> GIDPFTSTQQHTEPAEEETLHNIITDTENVQGSFSKHEFQAETKKLLDIVARSLYSEKEVFIRELISNGSDALEKLRHRMITAGGDTAPMEIHLQTDSVKGTFTIQDTGVGMNKEDLVSNLGTIARSGSKAFLDALQNQAEASSSIIGQFGVGFYSAFMVADKVEVYSQSAEADAPGYKWSSDGSGVFEVAEASGVRQGTKIVLHLKDDCKEFSSEDRVKEVVTKYSNFVSFPIFLNGRRLNTLQALWMMEPKDISEWQHEEFYRYVAQAYDKPRYTLHYRADAPLNIRSIFYVPEMKPSMFDVSREMGSSVALYSRKILIQTKATDILPKWLRFLRGVVDSEDIPLNLSRELLQESALIRKLRDVLQQRVIRFLLDQSKKDPEKYARFFEDYGLFMREGIVTTGEQSVKEDIAKLLRFESSALPAGQQTSLMEYSSRMKAGTRNIYYLCAPNRHLAEHSPYFEAMKQKDMEVLFCFEQFDELTLLHLREFDRKKLISAETDIVVDHYKEEKFQDSKPASERLSSEQAEDLLAWMRNALVQRVTNIKVTPRLDTHPAMITVLEMGAARHFLRTQQLARSSEERAQILQPTLEINTGHDLIKKLHALKDSNPELAQLLLEQIYDNAMIAAGLNEDPRPMISRLNQLLTRALEKHGSDSATHIKFSKRDEDGKELAGATMELRDSSGK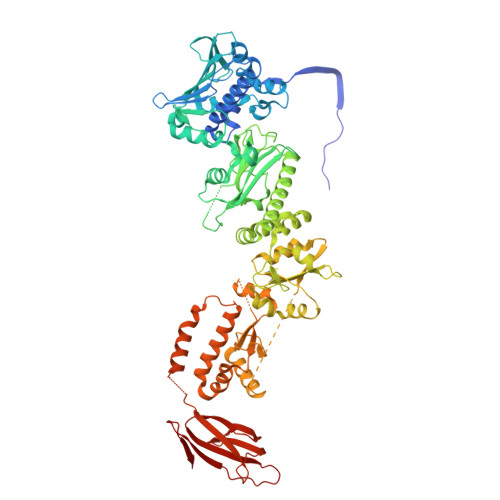TISTWISDGQVKDFYLYPGKYTFVETAAPDGYEVATAITFTVNEQGQVTVNG N-(4-methylphenyl)-N'-[(1P,2'P)-4-propoxy-5-propyl-2'-(1H-tetrazol-5-yl)[1,1'-biphenyl]-3-yl]urea 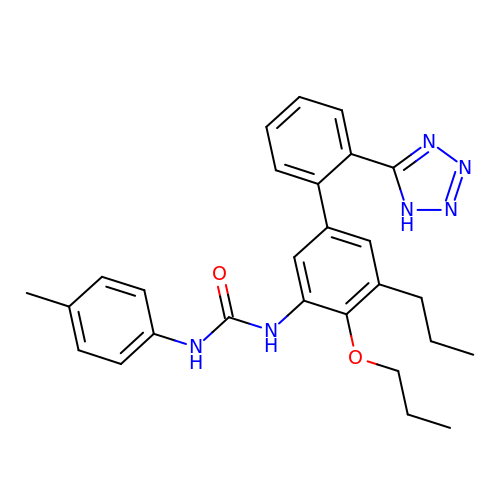| C27 H30 N6 O2 | UCPMUXOPKQHTIZ-UHFFFAOYSA-N> A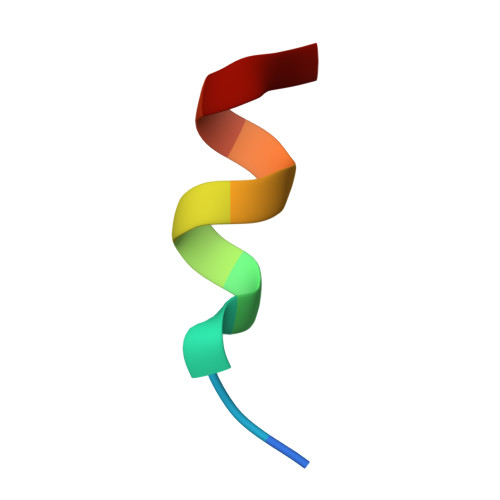HKILHRLLQE> MASMTGGQQMGRDLQVTLYGTIKAGVEVSRVKDAGTYKAQGGKSKTATQIADFGSKIGFKGQEDLGNGMKAIWQLEQKASIAGTNSGWGNRQSFIGLKGGFGTVRAGNLNTVLKDSGDNVNAWESGSNTEDVLGLGTIGRVESRE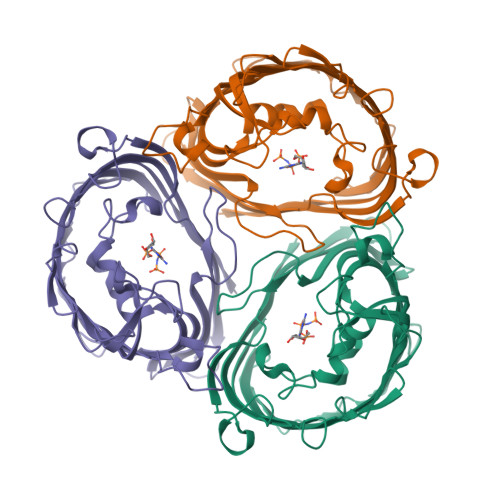ISVRYDSPVFAGFSGSVQYVPRDNANDVDKYKHTKSSRESYHAGLKYENAGFFGQYAGSFAKYADLNTDAERVAVNTANAHPVKDYQVHRVVAGYDANDLYVSVAGQYEAAKNNEVGSIKGKKHEQTQVAATAAYRFGNVTPRVSYAHGFKAKVNGVKDANYQYDQVIVGADYDFSKRTSALVSAGWLKQGKGAGKVEQTASMVGLRHKF>[2x]MTVGAVVVDHEGNVAAAVSSGGLALKHPGRVGQAALYGCGCWAENTGAHNPYSTAVSTSGCGEHLVRTILARECSHALQAEDAHQALLETMQNKFISSPFLASEDGVLGGVIVLRSCRCSAEPDSSQNKQTLLVEFLWSHTTESMCVGYMSA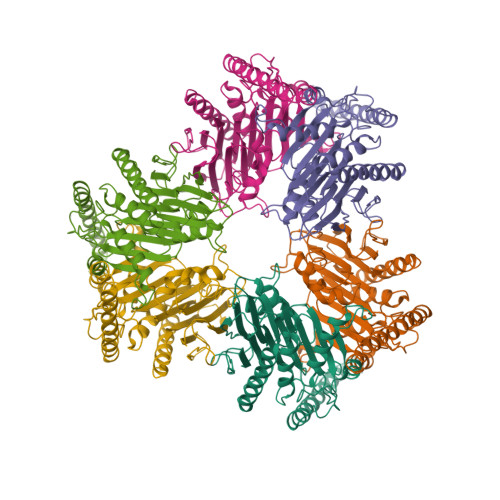QDGKAKTHISRLPPGAVAGQSVAIEGGVCRLEGSGSGGFVLVHAGAGYHSESKAKEYKHVCKRACQKAIEKLQAGALATDAVTAALVELEDSPFTNAGMGSNLNLLGEIECDASIMDGKSLNFGAVGALSGIKNPVSVANRLLCEGQKGKLSAGRIPPCFLVGEGAYRWAVDHGIPSCPPNIMTTRFSLAAFKRNKRKLELAERVDTDFMQLKKRRQSSEKENDSGTLDLEHHHHHH>[3x]SNLAIYWGQGPNQLRLSHFCQETSLDIINIGFINYFPDMSPGHWPGSNFGNQCDGSVYVTNDGVVTKLLSGCHQIMEDIPICQAAGKKVLLSIGGAYPPDQSILSEDSAVAFATFLWGAFGPVAEGWEGPRPFGDVVVDGFDFDIEHNGGFGYATMVNTFRQYFNQVPERKFYLSAAPQCIIPDAQLSDAIFNAAFDF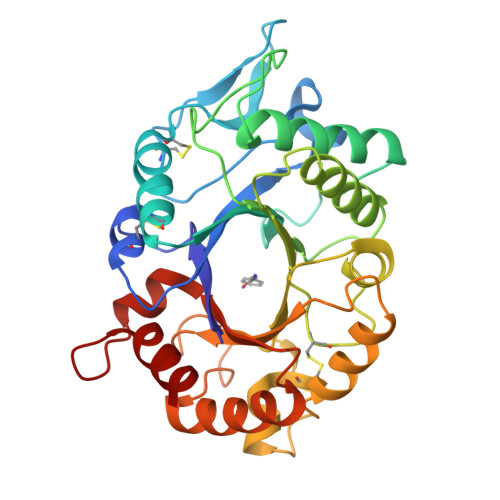IWIQYYNTAACSAKSFIDTSLGTFNFDAWVTVLKASASKDAKLYVGLPASETAANQGYYLTPDEVESLVSTYMDRYPDTFGGIMLWEATASENNQIDGAPYADHMKDILLH> GAGCAGACATGA;> CGTCACTCA;> TCAACG;> TCTGAGTGTGTCTGC

In this work, we exhaustively probe the ability of all 36 immobile HJ sequences to form DNA crystals in two different designed systems. Three separate self-assembling DNA crystal systems are described in this report: the “4 × 5” and “4 × 6” designs (collectively referred to as the 4 × N systems), and a third construct with a “scrambled” sequence variant of the 4 × 6 lattices. Self-assembly was mediated by three constituent oligonucleotides: (S1) containing four sequence repeats of either 5 or 6 bases; (S2) composed of 21 bases containing complementary regions to both (S1); and (S3) which forms the second junction crossover. The HJ serves as the fundamental component at the core of each unit, and the ultimate assembly of the full lattice is facilitated by the complementary 2-base sticky ends that tail each duplex.

In parallel, we employed the previously reported J1 4 × 6 system (3.05 Å), with P32 symmetry. Seventeen of the 36 junctions successfully crystallized, a 47% success rate. Unlike the 4 × 5 motif, nearly all of the 4 × 6 junction sequences had a strong preference for crystallization in buffers containing ≥2.0 M salts (e.g., LiCl, Li2SO4, KCl, and NaCl), with the majority preferring slightly basic pH conditions in cacodylic acid. The average cell constants for the P32 crystals were a = b = 68.29 Å c = 55.68 Å. The c-axis, in particular, was ~5 Å shorter, and had a much larger degree of variability (σ = 1.97), than those that crystallized using the 4 × 5 motif. The broad range of the short axis spanned from 52.77 to 60.36 Å, and we posit that the flexible axis lengths could be responsible for rendering a larger number of junctions fatal than the 4 × 5 system. However, in the majority of the crystal structures reported here, the cacodylate anion indeed fits best into the electron density map of our X-ray structures, due to the presence of sodium cacodylate in the crystallization solution.(1R)-1,2,2-TRIMETHYLPROPYL (R)-METHYLPHOSPHINATE | C7 H17 O2 P | 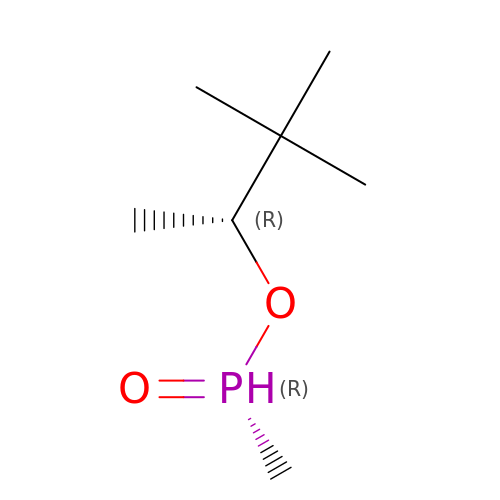QZUGWOMGKDLYKO-ZCFIWIBFSA-N> GAMA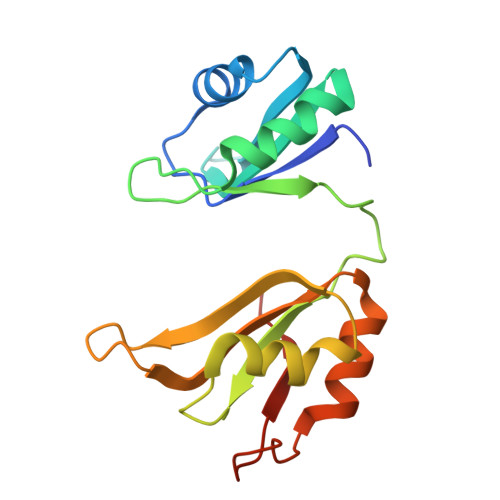SNTNLIVNYLPQDMTDRELYALFRAIGPINTCRIMRDYKTGYSFGYAFVDFTSEMDSQRAIKVLNGITVRNKRLKVSYARPGGESIKDTNLYVTNLPRTITDDQLDTIFGKYGSIVQKNILRDKLTGRPRGVAFVRYNKREEAQEAISALNNVIPEGGSQPLSVRLAEEHGK>[4x]NPAAEAEFNILLATDSYKVTHYKQYPPNTSKVYSYFECREKKTENSKLRKVKYEETVFYGLQYILNKYLKGKVVTKEKIQEAK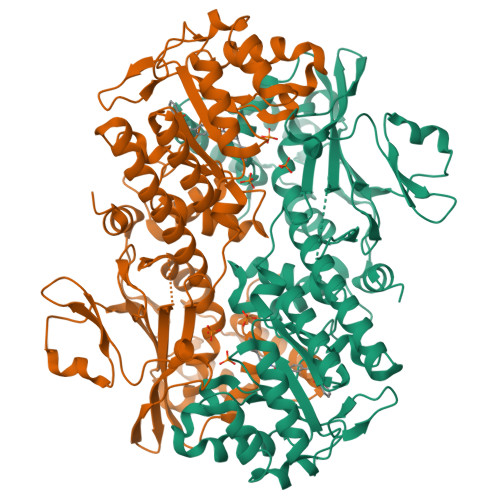DVYKEHFQDDVFNEKGWNYILEKYDGHLPIEIKAVPEGFVIPRGNVLFTVENTDPECYWLTNWIETILVQSWYPITVATNSREQKKILAKYLLETSGNLDGLEYKLHDFGYRGVSSQETAGIGASAHLVNFKGTDTVAGLALIKKYYGTKDPVPGYSVPAAEHSTITAWGKDHEKDAFEHIVTQFSSVPVSVVSDSYDIYNACEKIWGEDLRHLIVSRSTQAPLIIRPDSGNPLDTVLKVLEILGKKFPVTENSKGYKLLPPYLRVIQGDGVDINTLQEIVEGMKQKMWSIENIAFGSGGGLLQKLTRDLLNCSFKCSYVVTNGLGINVFKDPVADPNKRSKKGRLSLHRTPAGNFVTLEEGKGDLEEYGQDLLHTVFKNGKVTKSYSFDEIRKNAQLNIELEAAHHLEHHHHHHHH>[2x]EVVNIQTWINKPDVKHHFPCKEVKESGHMFPSHLLVT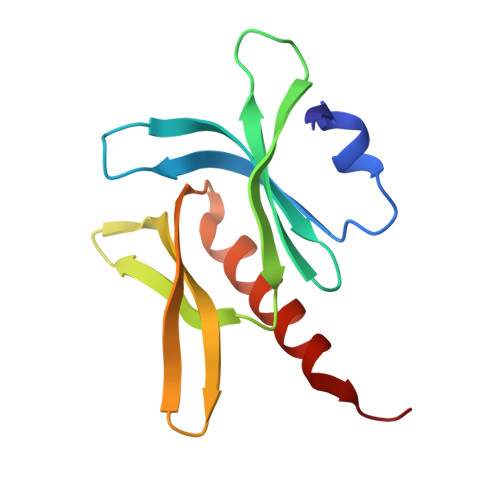ATHMYCLREIVSRKGLAYIQSRQALNSVVKITSKKKHPELITFKYGNSSASGIEILAIERYLIPNAGDATKAIKQQIMKVLDALES>[2x]MDERDALRISREIAGEVRKAIASMPLRERVKDVGMGKDGTPTKAADRVAEDAALEILRKERVTVVTEESGVLGEGDVFVALDPLDGTFNATQGIPVYSVSLCFSYSDKLKDAFFGYVYNLATGDEYYADSSGAYRNGERIEVSDAEELYCNAIIYYPDRKFPFERMRIFGSAATELCFFADGSFDCFLDIRPGKMLRIYDAAAGVFIAEKAGGKVTELD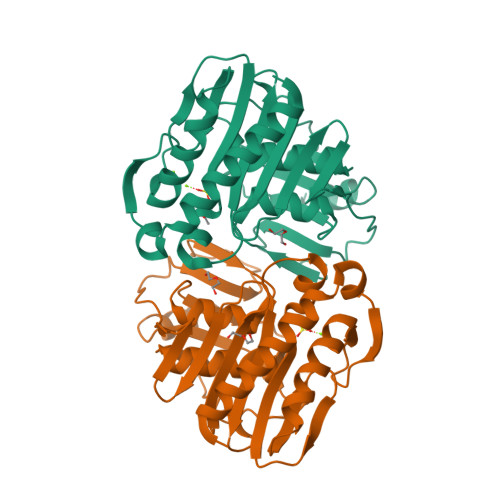GESLGNKKFDMQERLNIVAANEKLHPKLLELIK>[2x]SGSSEQELAAIVRDLGCGPYFLGTHDKRFPGFLAGNKLACAIVNTAGRETGGVHWLAFGWNPRSRTCYMFDPFGFSDRRLKQIYSFEYEAM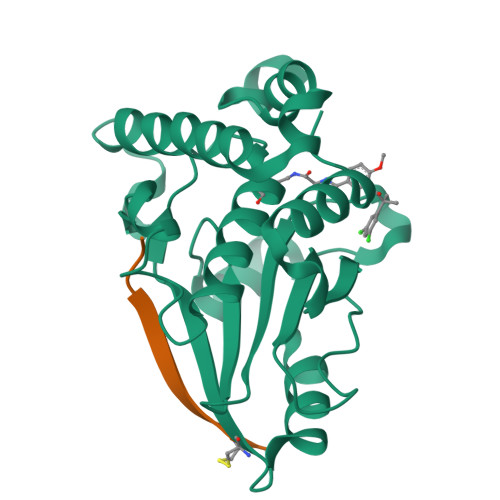LRRSALALSPDRCLSLEQSTQTVQGPDSAACGLFCCMFLHAFVHWPDRPMDGNPTMNLLTGVPNGMLQSPQVLPTLRRNQEKLYRFLAHHSPYFRSHRAAIEHATAFDKMKQL;>[2x]GVKSLKRRRCY>GPSPEIGQIVKIVKGRDRDQFSVIIKRVDDRFVYIADGDKRKVDRAKRKNMNHLKLIDHISPEVRHSFEETGKVTN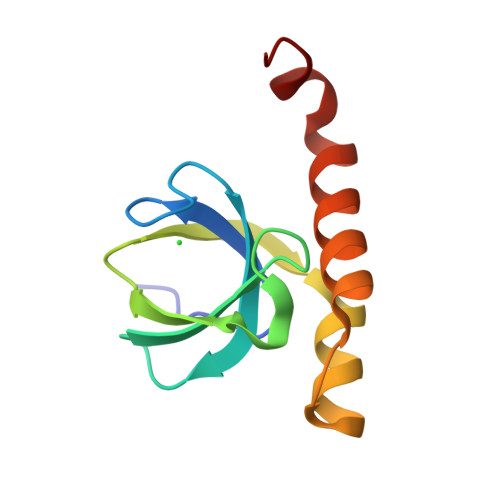GKLRFALKKFLEEHADLLKEGE[2x]> QRTGRSALAVLIRACYRLQQQLQRTRRALLHHSDAVLTSLHHVRM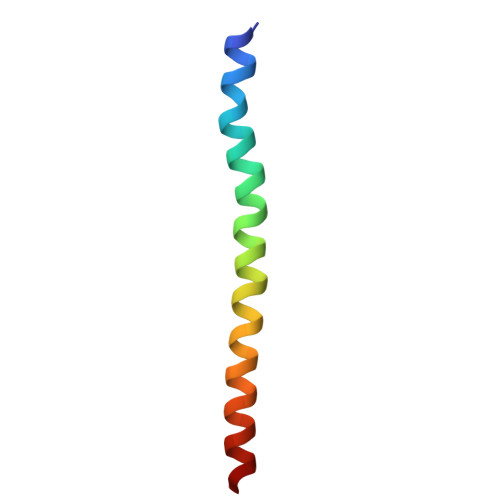LL(3S,5R,8R,9R,10R,12R,13R,14R,17S)-4,4,8,10,14-pentamethyl-17-[(2R)-2,6,6-trimethyloxan-2-yl]-2,3,5,6,7,9,11,12,13,15,16,17-dodecahydro-1H-cyclopenta[a]phenanthrene-3,12-diol 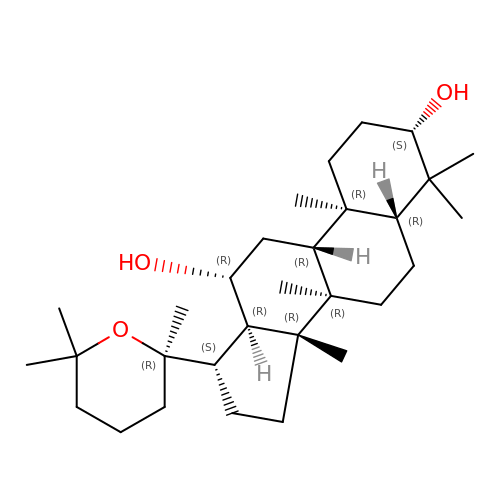| C30 H52 O3 | PVLHOJXLNBFHDX-XHJPDDKBSA-N> GHMRERYELSEKMLSACNLLKNTINDPKALTSKDMRFCLNTLQHEWFRVSSQKSAIPAMVGDYIAAFEAISPD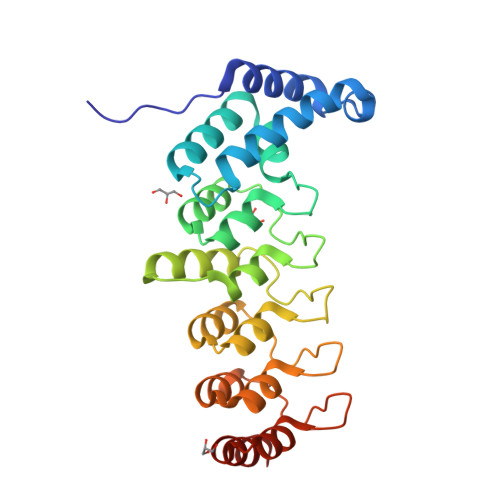VLRYVINLADGNGNTALHYSVSHSNFEIVKLLLDADVCNVDHQNKAGYTPIMLAALAAVEAEKDMRIVEELFGCGDVNAKASQAGQTALMLAVSHGRIDMVKGLLACGADVNIQDDEGSTALMCASEHGHVEIVKLLLAQPGCNGHLEDNDGSTALSIALEAGHKDIAVLLYAHVNFAKA>EGFIDDSTLTGGIYYWQRERDRKDVTDGDKYKTNLSHSTWNANLDFQSGYAADMFGLDIAAFTAIEMAENGDSSHPNEIAFSKSNKAYDEDWSGDKSGISLYKAAAKFKYGPVWARAGYIQPTGQTLLAPHWSFMPGTYQGAEAGANFDYGDAGALSFSYMWTNEYKAPWHLEMDEFYQNDKTTKVDYLHSFGAKYDFKNNFVLEAAFGQAEGYIDQYFAKASYKFDIAGSPLTTSYQFYGTRDKVDDRSVNDLYDGTAWLQALTFGYRAADVVDLRLEGTWVKADGQQGYFLQRMTPTYASSNGRLD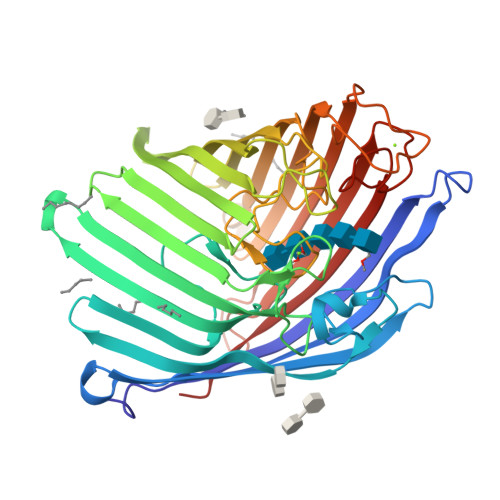IWWDNRSDFNANGEKAVFFGAMYDLKNWNLPGFAIGASYVYAWDAKPATWQSNPDAYYDKNRTIEESAYSLDAVYTIQDGRAKGTMFKLHFTEYDNHSDIPSWGGGYGNIFQDERDVKFMVIAPFTIF[2x]> ALPQTVRIGTDTTYAPFSSKDAKGEFIGFDIDLGNEMCKRMQVKCTWVASDADALIPSLKAKKIDAIISSLSITDKRQQEIAFSDKLYAADSRLIAAKGSPIQPTLESLKGKHVGVLQGSTQEAYANDNWRTKGVDVVAYANQDLIYSDLTAGRLDAALQDEVAASEGFLKQPAGKEYAFAGPSVKDKKYFGDGTGVGLRKDDTELKAAFDKALTELRQDGTYDKMAKKYF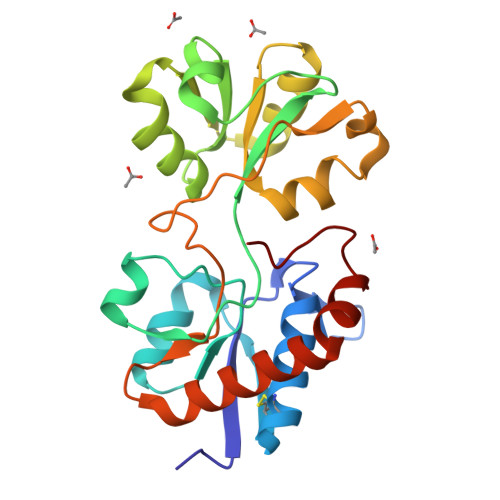DFNVYGD>GPGSMLRAANLDRSPEEYGMGSLDGRVVFITGAARGQGRSHAVMCAEQGANIVGVDICEDIDIVPYKLGTYEELEETARLVEKTGQEMLFRKADVRDKAVLQEVFDAGVEQFGHIDTVIANAGVVLTNPDERDASEALRLGLDIMLIGVWNTFQVAIPHMKERGQGGNLIATSSMIA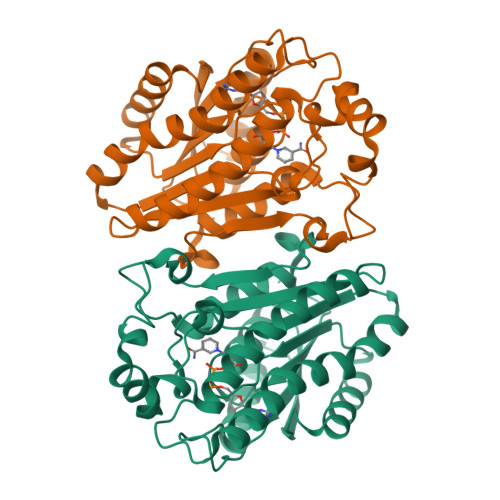LLDLTDGRGGTDAYLTSKLAITGLVRSYALMLAADRIRVNGVAPTNCSTPMITENPALFKVIEENPHLVNAMSTALPDFPMIEPRDVSNAILFLISDAGRSFTGSVLKVDAGMDVKR[2x]>MSVQVGVIMGS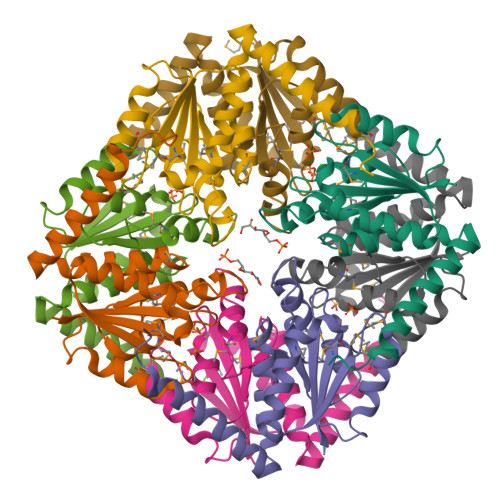KSDWSTMKECCDILDNLGIGYECEVVSAHRTPDKMFDYAETAKERGLKVIIAGAGGAAHLPGMVAAKTTLPVLGVPVKSSTLNGQDSLLSIVQMPAGIPVATFAIGMAGAKNAALFAASILQHTDINIAKALAEFRAEQTRFVLENPDPREH[8x]> MNL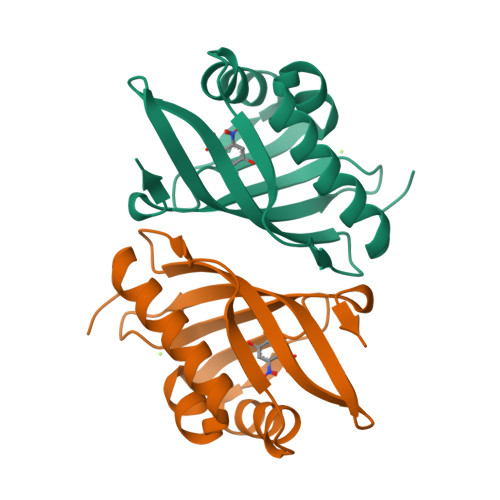PTAQEVQGLMARYIELVDVGDIEAIVQMYADDATVENPFGQPPIHGREQIAAFYRQGLGGGKVRACLTGPVRASHNGCGAMPFRVEMVWNGQPCALDVIDVMRFDEHGRIQTMQAYWSEVNLSVREPQ>GSHMADDPIAIVGMACRFPGGVHNPGELWEFIVGGGDAVTEMPTDRGWDLDALFDPDPQRHGTSYSRHGAFLDGAADFDAAFFGISPREALAMDPQQRQVLETTWELFENAGIDPHSLRGSDTGVFLGAAYQGYGQDAVVPEDSEGYLLTGNSSAVVSGRVAYVLGLEGPAVTVDTACSSSLVALHSACGSLRDGDCGLAVAGGVSVMAGPEVFTEFSRQGGLAVDGRCKAFSAEADGFGFAEGVAVVLLQRLSDARRAGRQVLGVVAGSAINQDGASNGLAAPSGVAQQRVIRKAWARAGITGADVAVVEAHGTGTRLGDPVEASALLATYGKSRGSSGPVLLGSVKSNIGHAQAAAGVAGVIKVVLGLNRGLVPPMLCRGERSPLIEWSSGGVELAEAVSPWPPAADGVRRAGVSAFGVSGTNAHVIIAEPPEPEPLPEPGPVGVLAAANSVPVLLSARTETALAAQARLLESAVDDSVPLTALASALATGRAHLPRRAALLAGDHEQLRGQLRAVAEGVAAPGATTGTASAGGVVFVFPGQGAQWEGMARGLLSVPVFAESIAECDAVLSEVAGFSASEVLEQRPDAPSL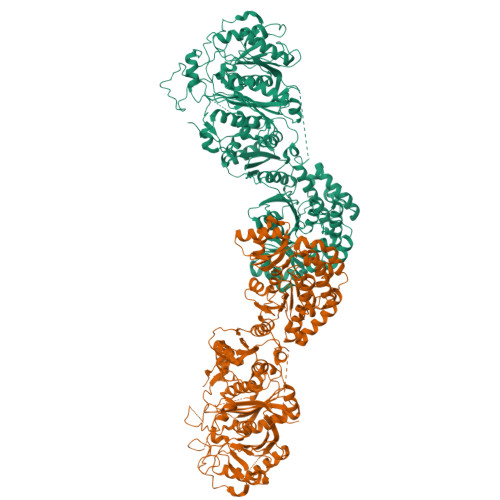ERVDVVQPVLFSVMVSLARLWGACGVSPSAVIGHSQGEIAAAVVAGVLSLEDGVRVVALRAKALRALAGKGGMVSLAAPGERARALIAPWEDRISVAAVNSPSSVVVSGDPEALAELVARCEDEGVRAKTLPVDYASHSRHVEEIRETILADLDGISARRAAIPLYSTLHGERRDGADMGPRYWYDNLRSQVRFDEAVSAAVADGHATFVEMSPHPVLTAAVQEIAADAVAIGSLHRDTAEEHLIAELARAHVHGVAVDWRNVFPAAPPVALPNYPFEPQRYWLQPEV[4x]>GMSTQENVQIVKDFFAAMGRGDKKGLLAVSAEDIEWIIPGEWPLAGTHRGHAALAALLQKASEMVEISYPEPPEFVAQGERVLVVGFATGRVKSTNRTFEDDWVFAITVRKSKVTSIREYIDTL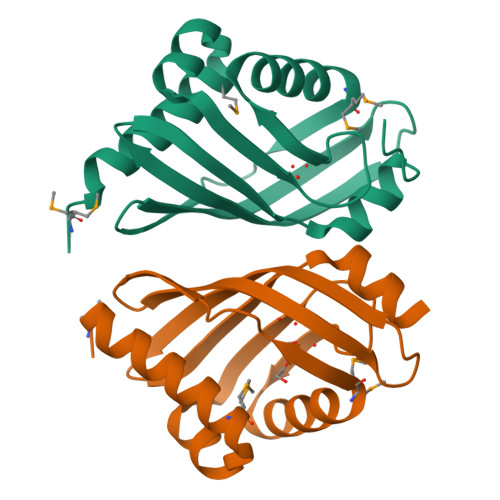ALARATNFNAT[2x]3'-amino-5-[5-amino-3-(4-hydroxyphenyl)-1H-pyrazol-4-yl][1,1'-biphenyl]-2-ol | C21 H18 N4 O2 | 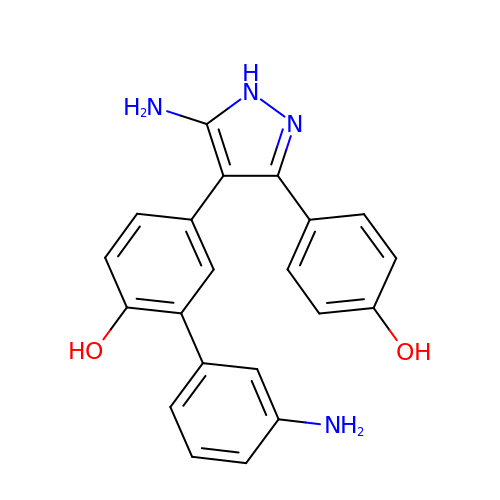YIPHDXIYQIAWDD-UHFFFAOYSA-N>[2x]MEFNESCPQI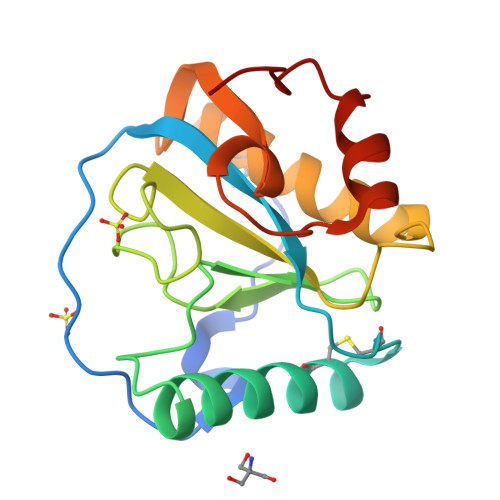IGRSEWTDVDAKSINYLIIPIPYVIIHHTVTAECNTRSECIAQAENIRSYHMDSNGWDDIGYSFLIGGDGNVYEGRGWNREGAHTIGYNKKSVGIGFIGNFQEKAASDKMLNAAHALIHCGKSKGILREDIRVIGAKQVTATMSPGSKLQKQIKNWLEWVPTP> MSSNNSGLSAAGEIDESLYSRQLYVLGKEAMLKMQTSNVLILGLKGLGVEIAKNVVLAGVKSMTVFDPEPVQLADLSTQFFLTEKDIGQKRGDVTRAKLAELNAYVPVNVLDSLDDVTQLSQFQVVVATDTVSLEDKVKINEFCHSSGIRFISSETRGLFGNTFVDLGDEFTVLDPTGEEPRTGMVSDIEPDGTVTMLDDNRHGLEDGNFVRFSEVEGLDKLNDGTLFKVEVLG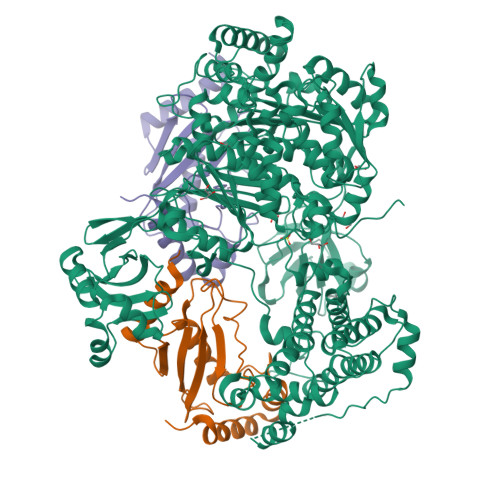PFAFRIGSVKEYGEYKKGGIFTEVKVPRKISFKSLKQQLSNPEFVFSDFAKFDRAAQLHLGFQALHQFAVRHNGELPRTMNDEDANELIKLVTDLSVQQPEVLGEGVDVNEDLIKELSYQARGDIPGVVAFFGGLVAQEVLKACSGKFTPLKQFMYFDSLESLPDPKNFPRNEKTTQPVNSRYDNQIAVFGLDFQKKIANSKVFLVGSGAIGCEMLKNWALLGLGSGSDGYIVVTDNDSIEKSNLNRQFLFRPKDVGKNKSEVAAEAVCAMNPDLKGKINAKIDKVGPETEEIFNDSFWESLDFVTNALDNVDARTYVDRRCVFYRKPLLESGTLGTKGNTQVIIPRLTESYSSSRDPPEKSIPLCTLRSFPNKIDHTIAWAKSLFQGYFTDSAENVNMYLTQPNFVEQTLKQSGDVKGVLESISDSLSSKPHNFEDCIKWARLEFEKKFNHDIKQLLFNFPKDAKTSNGEPFWSGAKRAPTPLEFDIYNNDHFHFVVAGASLRAYNYGIKSDDSNSKPNVDEYKSVIDHMIIPEFTPNANLKIQVNDDDPDPNANAANGSDEIDQLVSSLPDPSTLAGFKLEPVDFEKDDDTNHHIEFITACSNCRAQNYFIETADRQKTKFIAGRIIPAIATTTSLVTGLVNLELYKLIDNKTDIEQYKNGFVNLALPFFGFSEPIASPKGEYNNKKYDKIWDRFDIKGDIKLSDLIEHFEKDEGLEITMLSYGVSLLYASFFPPKKLKERLNLPITQLVKLVTKKDIPAHVSTMILEICADDKEGEDVEVPFITIHL;>[2x]GMASLPKRIIKETEKLVSDPVPGITAEPHDDNLRYFQVTIEGPEQSPYEDGIFELELYLPDDYPMEAPKVRFLTKIYHPNIDRLGRICLDVLKTNWSPALQIRTVLLSIQALLASPNPNDPLANDVAEDWIKNEQGAKAKAREWTKLYAKKKPE>[3x]NSAM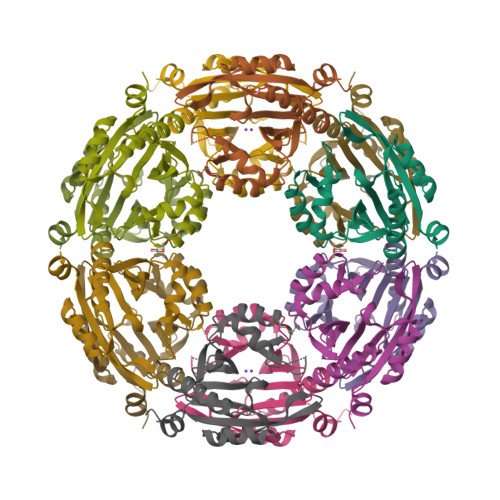STTSSVRLRPLEREDLPFVHQLDNNASIMRYWFEEPYEAFVELCDLYDKHIHDQSERRFIIESQGTKIGLVELVEINHIHRRAEFQIIIDPTHQGKGYAGAAAKLAMEYGFSVLNLYKLYLIVDKENEKAIHIYSKLGFEIEGELKQEFFINGEYRTVIRMCIFQPQYLAKYKTPSIKNA> FNCLPGWSAYDQHCYQAFNEPKTWDEAERFCTEQAKRGHLVSIGSDGEADFVAQLVTNNIKRPELYVWIGLRDRRKEQQCSSEWSMSASIIYVNWNTGE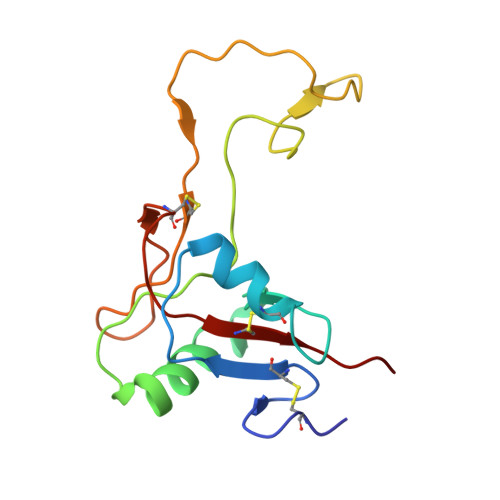SQMCQGLARWTGFRKWDYSDCQAKNPFVCKFSSEC> TQEIYPIKEANGRTRKALIICNTEFKHLSLRYGANFDIIGMKGLLEDLGYDVVVKEELTAEGMESEMKDFAALSEHQTSDSTFLVLMSHGTLHGICGTMHSEKTPDVLQYDTIYQIFNNCHCPGLRDKPKVIIVQAARGGNSGEMWIRESSKPQLCRGVDL;>TLKLCSPEEFTRLCREKTQEIYPIKEANGRTRKALIICNTEFKHLSLRYGANFDIIGMKGLLEDLGYDVVVKEELTAEGMESEMKDFAALSEHQTSDSTFLVLMSHGTLHGICGTMHSEKTPDVLQYDTIYQIFNNCHCPGLRDKPKVIIVQAARGGNSGEMWIRES[2x];>[3x]ADFQGLYAEVKACSSELESLEMELRQQILVNIGKILQDQPSMEALEASLGQGLCSGGQVEPLDGPAGCILECLVLDSGELVPELAAPIFYLLGALAVLSETQQQLLAKALETTVLSKQLELVKHVLEQSTPWQEQSSVSLPTVLLGDCWDEKNPTWVLLEECGLRLQVESPQVHWEPTSLIPTSALYASLFLLSSLGQ;>[7x]DFQGLYAEVKACSSELESLEMELRQQILVNIGKILQDQPSMEALEASLGQGLCSGGQVEPLDGPAGCILECLVLDSGELVPELAAPIFYLLGALAVLSETQQQLLAKALETTVLSKQLELVKHVLEQSTPWQEQSSVSLPTVLLGDCWDEKNPTWVLLEECGLRLQVESPQVHWEPTSLIPTSALYASLFLLSSLGQ;>TLKLCSPEEFTRLCREKTQEIYPIKEANGRTRKALIICNTEFKHLSLRYGANFDIIGMKGLLEDLGYDVVVKEELTAEGMESEMKDFAALSEHQTSDSTFLVLMSHGTLHGICGTMHSEKTPDVLQYDTIYQIFNNCHCPGLRDKPKVIIVQAARGGNSGEMWIRE[4x];> AEVKACSSELESLEMELRQQILVNIGKILQDQPSMEALEASLGQGLCSGGQVEPLDGPAGCILECLVLDSGELVPELAAPIFYLLGALAVLSETQQQLLAKALETTVLSKQLELVKHVLEQSTPWQEQSSVSLPTVLLGDCWDEKNPTWVLLEECGLRLQVESPQVHWEPTSLIPTSALYASLFLLSSLGQ;>LKLCSPEEFTRLCREKTQEIYPIKEANGRTRKALIICNTEFKHLSLRYGANFDIIGMKGLLEDLGYDVVVKEELTAEGMESEMKDFAALSEHQTSDSTFLVLMSHGTLHGICGTMHSEKTPDVLQYDTIYQIFNNCHCPGLRDKPKVIIVQAARGGNSGEMWIRE[5x];> TQEIYPIKEANGRTRKALIICNTEFKHLSLRYGANFDIIGMKGLLEDLGYDVVVKEELTAEGMESEMKDFAALSEHQTSDSTFLVLMSHGTLHGICGTMHSEKTPDVLQYDTIYQIFNNCHCPGLRDKPKVIIVQAARGGNSGEMWIRE;>[3x]LSLLSDGIDEEELIEAADFQGLYAEVKACSSELESLEMELRQQILVNIGKILQDQPSMEALEASL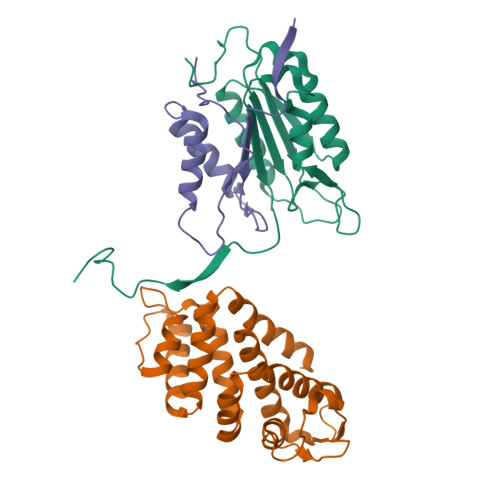GQGLCSGGQVEPLDGPAGCILECLVLDSGELVPELAAPIFYLLGALAVLSETQQQLLAKALETTVLSKQLELVKHVLEQSTPWQEQSSVSLPTVLLGDCWDEKNPTWVLLEECGLRLQVESPQVHWEPTSLIPTSALYASLFLLSSLGQ;>[2x]TQEIYPIKEANGRTRKALIICNTEFKHLSLRYGANFDIIGMKGLLEDLGYDVVVKEELTAEGMESEMKDFAALSEHQTSDSTFLVLMSHGTLHGICGTMHSEKTPDVLQYDTIYQIFNNCHCPGLRDKPKVIIVQAARGGNSGEMWIRES;> TLKLCSPEEFTRLCREKTQEIYPIKEANGRTRKALIICNTEFKHLSLRYGANFDIIGMKGLLEDLGYDVVVKEELTAEGMESEMKDFAALSEHQTSDSTFLVLMSHGTLHGICGTMHSEKTPDVLQYDTIYQIFNNCHCPGLRDKPKVIIVQAARGGNSGEMWIR;> AADFQGLYAEVKACSSELESLEMELRQQILVNIGKILQDQPSMEALEASLGQGLCSGGQVEPLDGPAGCILECLVLDSGELVPELAAPIFYLLGALAVLSETQQQLLAKALETTVLSKQLELVKHVLEQSTPWQEQSSVSLPTVLLGDCWDEKNPTWVLLEECGLRLQVESPQVHWEPTSLIPTSALYASLFLLSSLGQ;> FQGLYAEVKACSSELESLEMELRQQILVNIGKILQDQPSMEALEASLGQGLCSGGQVEPLDGPAGCILECLVLDSGELVPELAAPIFYLLGALAVLSETQQQLLAKALETTVLSKQLELVKHVLEQSTPWQEQSSVSLPTVLLGDCWDEKNPTWVLLEECGLRLQVESPQVHWEPTSLIPTSALYASLFLLSSLGQ;>AVKLSHVEKDFIAFYSTTPHHLSYRDKTGGSYFITRLISCFRKHACSCHLFDIFLKVQQSFEKASIHSQMPTIDRATLTRYFYLFPGN[15x];> VKLSHVEKDFIAFYSTTPHHLSYRDKTGGSYFITRLISCFRKHACSCHLFDIFLKVQQSFEKASIHSQMPTIDRATLTRYFYLFPGN>NTIQQLMMILNSASDQPSENLISYFNNCTVNPKESILKRVKDIGYIFKEKFAKAVGAGCVAIGSQRYKLGVRLYYRVMESMLKSEEERLSIQNFSKLLNDNIFHMSLLACALEVVMATYSRSTSQNLDSGTDLSFPWILNVLNLKAFDFYKVIESFIKAEGNLTREMIKHLERCEHRIMESLAWLSDSPLFDLIKQSKTREGKSTSLSLFYKKVYRLAYLRLNTLCERLLSEHPELEHIIWTLFQHTLQNEYELMRDRHLD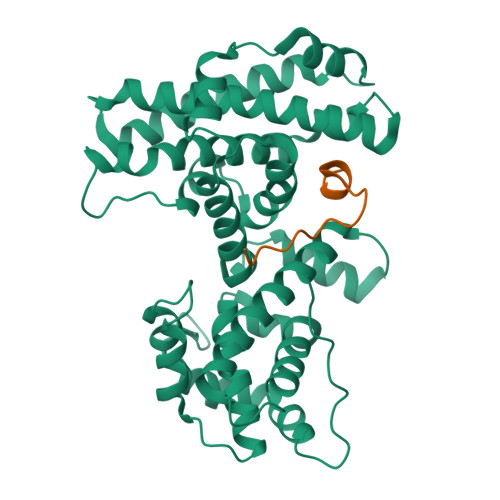QIMMCSMYGICKVKNIDLKFKIIVTAYKDLPHAVQETFKRVLIKEEEYDSIIVFYNSVFMQRLKTNILQYASTRPPTLSPIPHI[2x];>DDYLWGLEAGEGISDLFD[3x]>[4x]AADVYVPDEWEVAREKITMSRELGQGSFGMVYEGVAKGVVKDEPETRVA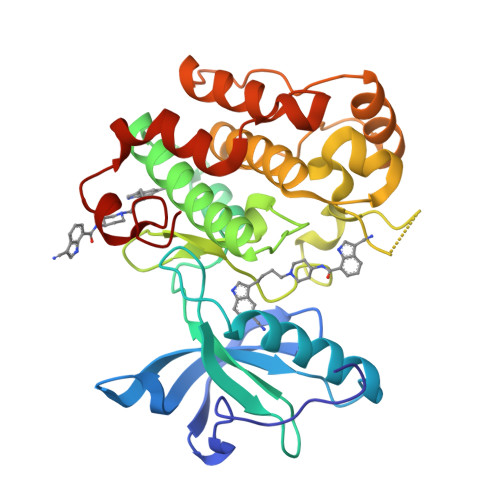IKTVNEAASMRERIEFLNEASVMKEFNCHHVVRLLGVVSQGQPTLVIMELMTRGDLKSYLRSLRPAMANNPVLAPPSLSKMIQMAGEIADGMAYLNANKFVHRDLAARNCMVAEDFTVKIGDFGMTRDIYETDYYRKGGKGLLPVRWMSPESLKDGVFTTYSDVWSFGVVLWEIATLAEQPYQGLSNEQVLRFVMEGGLLDKPDNCPDMLFELMRMCWQYNPKMRPSFLEIISSIKEEMEPGFREVSFYYSEENK> MATSGFSKPLHYPPVRRDETVVDDYFGVKVADPYRWLEDPNSEETKEFVDNQEKLANSVLEECELIDKFKQKIIDFVNFPRCGVPFRRANKYFHFYNSGLQAQNVFQMQDDLDGKPEVLYDPNLREGGRSGLSLYSVSEDAKYFAFGIHSGLTEWVTIKILKTEDRSYLPDTLEWVKFSPAIWTHDNKGFFYCPYPPLKEGEDHMTRSAVNQEARYHFLGTDQSEDILLWRDLENPAHHLKCQITDDGKYFLLYILDGCDDANKVYCLDLTKLPNGLESFRGREDSAPFMKLIDSFDASYTAIANDGSVFTFQTNKDAPRKKLVRVDLNNPSVWTDLVPESKKDLLESAHAVNENQLILRYLSDVKHVLEIRD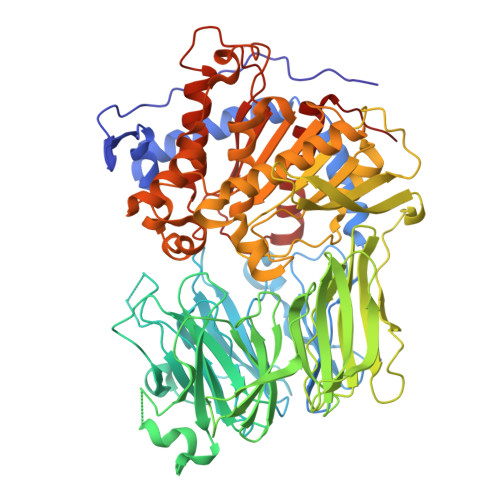LESGALQHRLPIDIGSVDGITARRRDSVVFFKFTSILTPGIVYQCDLKNDPTQLKIFRESVVPDFDRSEFEVKQVFVPSKDGTKIPIFIAARKGISLDGSHPCEMHGYGGFGINMMPTFSASRIVFLKHLGGVFCLANIRGGGEYGEEWHKAGFRDKKQNVFDDFISAAEYLISSGYTKARRVAIEGGANGGLLVAACINQRPDLFGCAEANCGVMDMLRFHKFTLGYLWTGDYGCSDKEEEFKWLIKYSPIHNVRRPWEQPGNEETQYPATMILTADHDDRVVPLHSFKLLATMQHVLCTSLEDSPQKNPIIARIQRKAAHYGRATMTQIAEVADRYGFMAKALEAPWID>[2x]MAETDGSIPLIPVRMLNEHVYCPRLAYLMWVQGEFSHNEFTVDGVIRHRRVDAGGGVLPSETQEDSRIHARSVSLSSERLGITAKIDLVEGEGAYVSPVDYKRGKRPHVAGGAYEPERVQLCAQGLLLREHGFASDGGALYFVASRERVPVAFDDELIGRTLAAIDEMGRTALSGTMPPPLEDSPKCPRCSLVGICLPDEVRFLSHLSVEPRPIIPADGRGLPLYVQSPKAYVRKDGDCLVIEEERVRVAEARLGETSQVALFGNATLTTAALHECLRREIPVTWLSYGGWFMGHTVSTGHRNVETRTYQYQRSFDPETCLNLARRWIVAKIANCRTLLRRNWRGEGDEAKAPPGLLMSLQDDMRHAMRAPSLEVLLGIEGASAGRYFQHFSRMLRGGDGEGMGFDFTTRNRRPPKDPVNALLSFAYAMLTREWTVALAAVGLDPYRGFYHQPRFGRPALALDMMEPFRPLIADS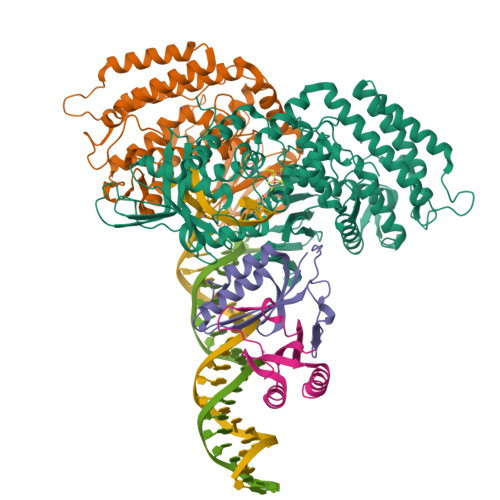TVLMAINNGEIRTGDFVRSAGGCNLTDSARKRFIAGFERRMEQEVTHPIFKYTISYRRLLEVQARLLTRYLSGEIPAYPNFVTR;>MEHLYIVSYDIRNQRRWRRLFKTMHGFGCWLQLSVFQCRLDRIRIIKMEAAINEIVNHAEDHVLILDLGPAENVKPKVSSIGKTFDPILRQAVIV[2x]>GAMDPMKAKRVQAKIEMEFPSEDVAKVVYEAVLYEHLSVPYRRSEIDFKLEGKKIILDIKATDSSA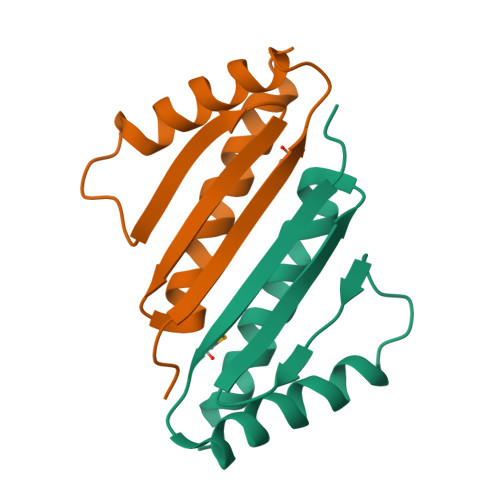LRGTVNSYLRWIKAAIDVIEV[2x]>MRGSHHHHHHGSMEQSHQNLQSQFFIEHILQILPHRYPMLLVDRITELQANQKIVAYKNITFNEDVFNGHFPNKPIFPGVLIVEGMAQSGGFLAFTSLWGFDPEIAKTKIVYFMTIDKVKFRIPVTPGDRLEYHLEVLKHKGMIWQVGGTAQVDGKVVAEAELKAMI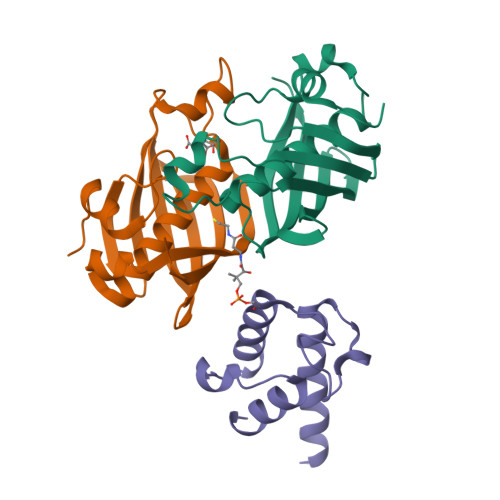AERE[2x];> GTSSMGYLMALFEDIQAVIAEQLNVDAAQVTPEAEFVKDLGADSLDVVELIMALEEKFGIEIPDEQAEKIVNVGDVVKYIEDNKLA>GSHNDKDLSTWQTFRRLWPTIAPFKAGLIVAGVALILNAASDTFMLSLLKPLLDDGFGKTDRSVLVWMPLVVIGLMILRGITSYVSSYCISWVSGKVVMTMRRRLFGHMMGMPVSFFDKQSTGTLLSRITYDSEQVASSSSGALITVVREGASIIGLFIMMFYYSWQLSIILIVLAPIVSIAIRVVSKRFRNISKNMQNTMGQVTTSAEQMLKGHKEVLIFGGQEVETKRFDKVSNRMRLQGMKMVSASSISDPIIQLIASLALAFVLYAASFPSVMDSLTAGTITVVFSSMIALMRPLKSLTNVNAQFQRGMAACQTLFTILDSEQEKDEGKRVIERATGDVEFRNVTFTYPGRDVPALRNINLKIPAGKTVALVGRSGSGKSTIASLITRFYDIDEGEILMDGHDLREYTLASLRNQVALVSQNVHLFNDTVANNIAYARTEQYSREQIEEAARMAYAMDFINKMDNGLDTVIGENGVLLSGGQRQRIAIARALLRDSPILILDEATSALDTESERAIQAALDELQKNRTSLVIAHRLSTIEKADEIVVVEDGVIVERGTHNDLLEHRGVYAQLHKMQFGQ[2x]

The ATP-binding cassette (ABC) transporter, MsbA, plays a pivotal role in lipopolysaccharide (LPS) biogenesis by facilitating the transport of the LPS precursor lipooligosaccharide (LOS) from the cytoplasmic to the periplasmic leaflet of the inner membrane. MsbA forms a homodimer and exhibits a topology similar to other ABC transporters, comprising two NBDs and two transmembrane domains (TMDs) containing 12 transmembrane helices. Upon binding ATP, MsbA undergoes dimerization of the NBDs, inducing rearrangement in the TMDs. An ATP hydrolysis-driven conformational change promotes the transition to an outward-facing (OF) conformation, facilitating the flipping of LOS to the periplasmic side of the inner membrane for further modifications.

MsbA (78 µM) solubilized in C10E5 was prepared in the presence of 2.5-fold molar excess of KDL (194 µM) and incubated in the presence of 1 mM ATP and Mg2+. Four of the structures, ranging from 3.6 to 3.9 Å resolution, adopt open, inward-facing conformations (OIF) that vary in their degree of openness. a–d MsbA can adopt open, inward-facing conformations that are dynamic and vary in their degree of openness.> DYRSPFIASVSDQHGVVYITENKNKTVVIPCLGSISNLNVSLCARYPEKRFVPDGNRISWDSKK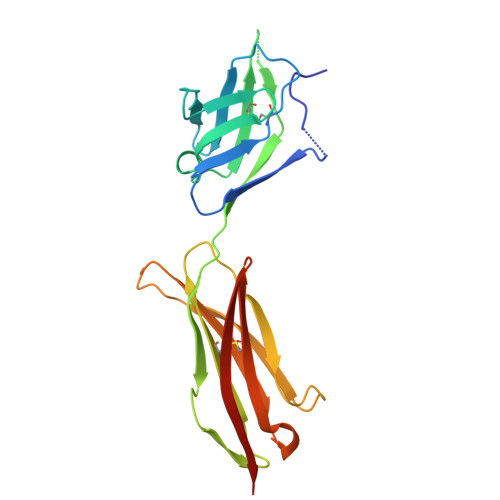GFTIPSYMISYAGMVFCEAKINDESYQSIMYIVVVVGYRIYDVVLSPSHGIELSVGEKLVLNCTARTELNVGIDFNWEYPSSKHQHKKLVNRDLKTQSGSEMKKFLSTLTIDGVTRSDQGLYTCAASSGLMTKKNSTFVRVHEDPIEGR(6S)-2-amino-3,6-dimethyl-6-[(1R,2R)-2-phenylcyclopropyl]-5,6-dihydropyrimidin-4(3H)-one | C15 H19 N3 O | 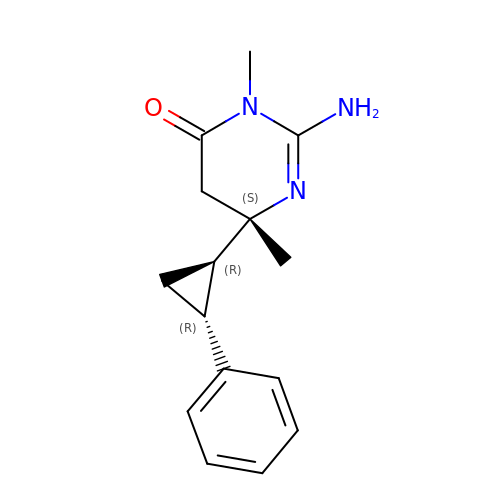YBXYDJCRBQOXMI-ZOWXZIJZSA-N>[2x]MGKSMTFKVGMKYMFKNKNSRKYLDISGNQTGNNANVQQYEYLADAPSERFFLHPLDNNYYAMINLNSGKVIDISGNQTSNNANIQQYEWLGDAPSEYWYFHREADGHYVIESKHSGKVLDIEGNQTGNNANVQQYEYLADAPSERFAVEEAGSVSLPSINTQPLSPVPQYETINDQLPEETERVVTAFTIVPAISVKDPHYGGDTAKQIKENPYYMVVKKQWWKKQESYVLAPSERYDFVTTTGIR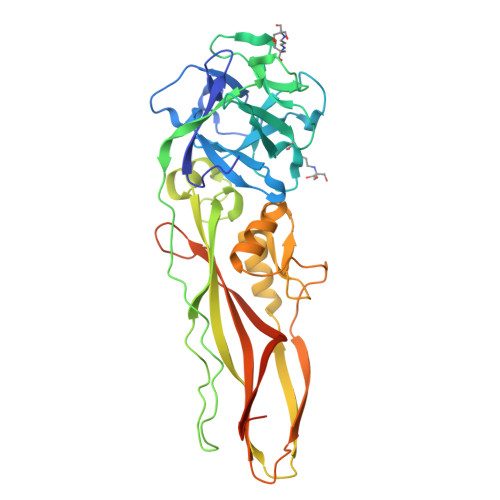VTDQETATKTVSWSIGADMGFSFKGFSMGMSSQYSQELQTSISHTTEQLKEETQEHHVTNPFLERMAYSRYILVTEYYVQRKNGTIVNAPWTMTDKTNAHAVTFPKSTGDLLNESTRKISKSESVK>GPSSPSLLRAIPGIAWIALLLLVIFYVFAVMGTKLFAQSFPEWFGTLGASMYTLFQVMTL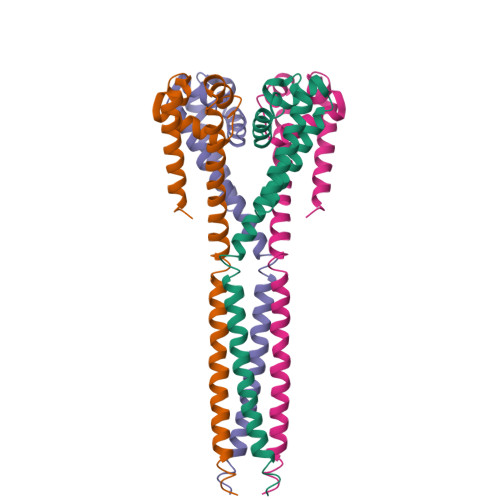ESWSMGIARPVIEAYPWAWIYFVSFILVSSFTVLNLFIGIIIESMQSAGWEAEDAKRIEQEQRAHDERLEMLQLIRDLSSKVDRLERRSGKR[4x]4-(2-[(6-methoxypyridin-3-yl)amino]-5-{[4-(methylsulfonyl)piperazin-1-yl]methyl}pyridin-3-yl)-6-methyl-1,3,5-triazin-2-amine | C21 H27 N9 O3 S | 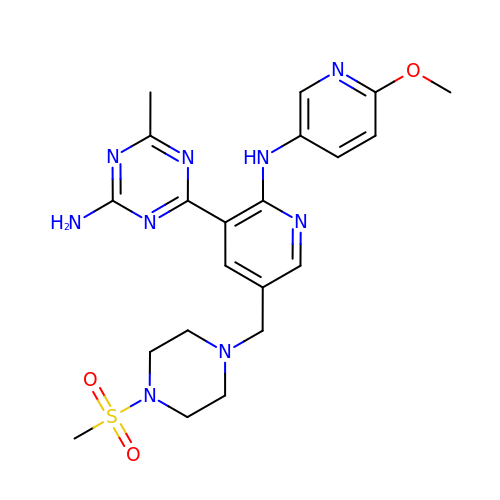RNTFRUPRTOCGJO-UHFFFAOYSA-N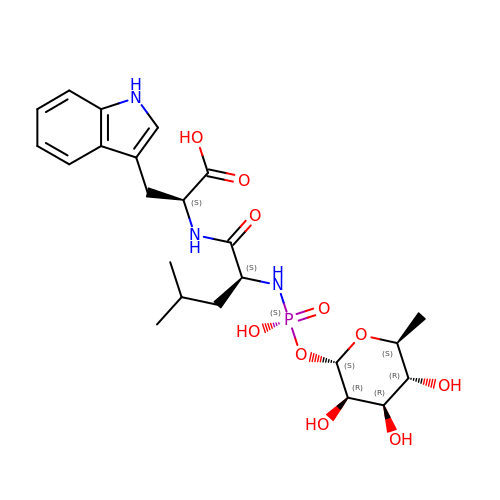N-ALPHA-L-RHAMNOPYRANOSYLOXY(HYDROXYPHOSPHINYL)-L-LEUCYL-L-TRYPTOPHAN | C23 H34 N3 O10 P | ZPHBZEQOLSRPAK-XLCYBJAPSA-N> NFTLKF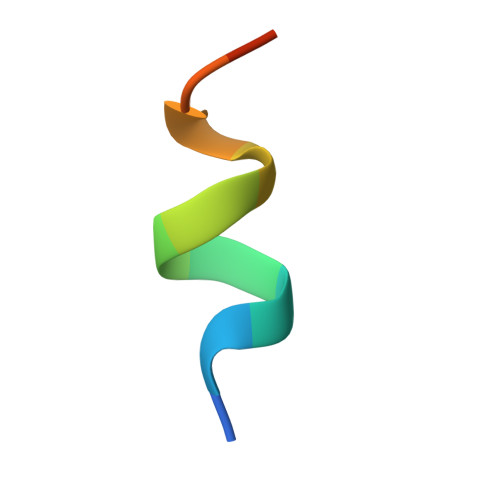WDIFRK> MEKDGLCRADQQYECVAEIGEGAYGKVFKARDLKNGGRFVALKRVRVQTGEEGMPLSTIREVAVLRHLETFEHPNVVRLFDVCTVSRTDRETKLTLVFEHVDQDLTTYLDKVPEPGVPTETIKDMMFQLLRGLDFLHSHRVVHRDLKPQNILVTSSGQIKLADFGLARIYSFQMALTSVVVTLWYRAPEVLLQSSYATPVDLWSVGCIFAEMFRRKPLFRGSSDVDQLGKILDVIGLPGEEDWPRDVALPRQAFHSKSAQPIEKFVTDIDELGKDLL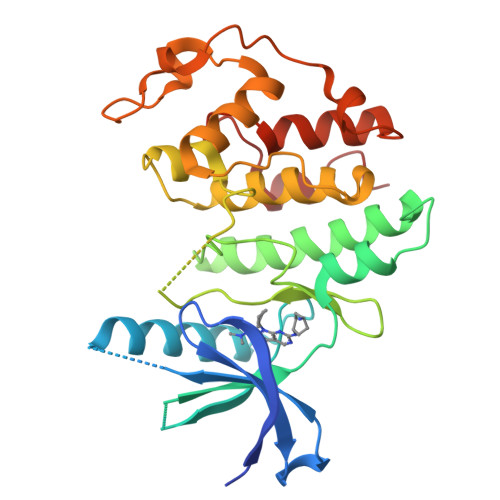LKCLTFNPAKRISAYSALSHPYFQ Toxoplasma gondii is one of the most significant parasites that impacts human health, with estimates that as many as one third to one half of the human population are infected. At the Center for Structural Genomics of Infectious Diseases (CSGID), the first Toxoplasma Structural Genomics Pipeline was established. The enzymes selected from the TDR database as small and tractable for expression and crystallization included: phosphoglycerate mutase II (hereafter referred to as PGM), nucleotide diphosphate kinase (NDK), ribulose phosphate 3-epimerase (RPE), ribose-5-phosphate isomerase (RPI), and ornithine aminotransferase (OAT). The genes encoding these enzymes were cloned, proteins expressed and purified, crystallized, and crystal structures were determined.

Phosphoglycerate mutase II, an enzyme at the core of the glycolytic pathway, catalyzes the transition from 3-phosphoglycerate to 2-phosphoglycerate, an important preparatory step upstream of enolase and pyruvate kinase. The P21212 asymmetric unit comprises four PGM chains [~0.4 Å root-mean-square-deviation (r.m.s.d.) over 240 Cα atoms] assembled in two dimers with BSA of ~1,900 Å2, while four chains bury a surface area of ~ 6,800 Å2. Eleven salt bridges, 15 hydrogen-bonded and 236 van der Waals interactions hold the tetramer in place. A sodium ion-binding site (e.g., NA 301/A) was identified during structure refinement. Tyr155, Val158, and Asn160 coordinate NA 301/A. Residues 12–257 (chain A), 15–259 (chain B), 15–257 (chain C), and 17–248 (chain D) are present in the deposited structure. TgPGM has an α/β/α-sandwich domain that comprises residues 12–107 and 169–257. Lys115 and Arg132 of this motif comprise a portion of the active site and together with Arg25, His26, Asn32, Thr38, Glu104, Tyr107, His199, and Asn201of the α/β/α domain shape the entrance to the active site. An interesting feature of the structure is a “scorpion tail” segment (residues 136–168 belonging to 310-helices η3, η4, and η5) that lies on top of the α/β/α domain. The tip of the tail possesses the sodium ion-binding site. With the present crystal structure, further structure-based molecular design approaches (such as virtual screening) is possible given the favorable SiteMap score (0.98).

>[4x]MFPASTFRRFFGNMAKAKYTLVLIRHGESTWNKENRFTGWTDVPLSPVGEQEAVEAAKALKEKGFEFDVAYTSVLQRAVVTCWTVLKGTDMCHIPVKSSWRLNERHYGALQGLNKAETAAKHGDEQVKIWRRSYDIPPPPLEKSDKRWPGNDAVYKMVPNEALPLTECLKDTVERVLPFWFDHIAPSIMEGKRVLVAAHGNSLRGLVKHLDKMSDEAVLELNIPTGVPLVYELDEDLQPVRHYYLLDEAELKAKMEAVANQGKAKGENLYFQSAGHHHHHH However, the most common paralogue OCP1 relies on an allosteric regulation for photo-recovery: OCP1 interacts with the fluorescence recovery protein (FRP), a small, dimeric regulator that terminates the interaction with the phycobilisome, and strongly accelerates the back-conversion of OCPR into the resting orange state. We show that this interaction between the orange carotenoid protein (OCP) and its unrelated regulator, the fluorescence recovery protein (FRP), evolved when a precursor of FRP was horizontally acquired by cyanobacteria. Homologues of FRP (termed FRP-like, FRPL) can also be found in distantly related bacteria, mainly proteobacteria and acidobacteria, suggesting an origin far beyond cyanobacteria.

To understand the ancestral state of FRPL proteins before they were transferred into cyanobacteria, we heterologously expressed, purified and characterized the FRPL from one of the few isolated, mesophilic bacteria that feature FRPL (PbFRPL): the gamma-proteobacterium Pseudomonas borbori, a close relative of P. aeruginosa. Circular dichroism spectroscopy of PbFRPL showed the typical all alpha-helical fold, previously found in FRP in solution, and native mass spectrometry confirmed the distinctive dimeric state. We solved PbFRPL’s crystal structure to a resolution of 1.8 Å. The N-terminal domain consists of two antiparallel alpha-helices of about 50 Å in length and features a homo-dimerization interface similar to those in FRPs with an estimated buried surface of around 675 Å2. In P. borbori, the frpl gene is encoded on its single chromosome, and we did not find any OCP, HCP or CTDH homologues. Epi-fluorescence microscopy of PbFRPL fused to an mVenus fluorophore and expressed from a plasmid under its native promotor in P. borbori showed a homogeneous distribution across the whole cell during exponential growth and an additional concentration at the cell poles upon starvation with increased whole-cell integrated fluorescence by about 2.5- to 3.4-fold above wild-type increase. Our data indicate that despite their extremely similar structures, FRPLs carry out a potentially stress-related function that must be totally unrelated to OCPs and the regulation of photoprotection. FRPL from P. borbori, Methylocaldum sp. and Chlorobi sp. had virtually no effect on OCP1’s photo-recovery. In our AlphaFold2 model, phenylalanine 76, lysine 102 and leucine 106 in FRP of Synechocystis sp. PCC 6803 are in contact with OCP1. P. borbori FRPL for instance has the phenylalanine, but features a tyrosine at position 102 and a serine at position 106.

> MHHHHHHMHDLKWSAAEKKLAHHVFEAALTTELAEIMADFKARAAAITQPQEIWPLQEYLARKQREIDRKYDYRYSQLLFVFGQLIREERVQEAQLAGLSEEKLGYIRRSASL> MSQRITIDPVTRIEGHLRIDCEIENGVVSKAWASGTMWRGMEEIVKNRDPRDAWMIVQRICGVCTTTHALSSVRAAESALNIDVPVNAQYIRNIILAAHTTHDHIVHFYQLSALDWVDITSALQADPTKASEMLKGVSTWHLNSPEEFTKVQNKIKDLVASGQLGIFANGYWGHPAMKLPPEVNLIAVAHYLQALECQRDANRVVALLGGKTPHIQNLAVGGVANPINLDGLGVLNLERLMYIKSFIDKLSDFVEQVYKVDTAVIAAFYPEWLTRGKGAVNYL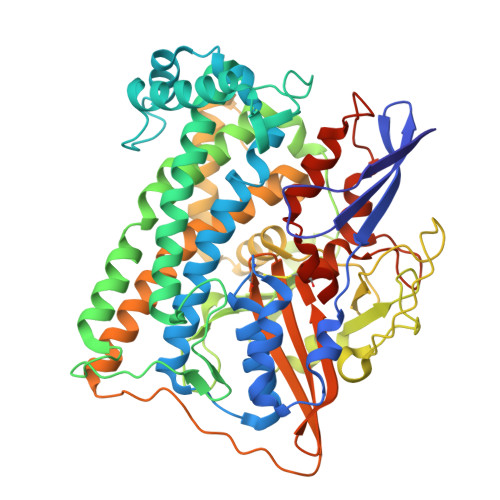SVPEFPTDSKNGSFLFPGGYIENADLSSYRPITSHSDEYLIKGIQESAKHSWYKDEAPQAPWEGTTIPAYDGWSDDGKYSWVKSPTFYGKTVEVGPLANMLVKLAAGRESTQNKLNEIVAIYQKLTGNTLEVAQLHSTLGRIIGRTVHCCELQDILQNQYSALITNIGKGDHTTFVKPNIPATGEFKGVGFLEAPRGMLSHWMVIKDGIISNYQAVVPSTWNSGPRNFNDDVGPYEQSLVGTPVADPNKPLEVVRTIHSFDPCMACAVHVVDADGNEVVSVKVL> SNAMSARKLFYLGPQGTFTHQAAVNAAQELARFEPQGFDLMPMDDVPQILDAAQHGDGWGIVAWENNVEGYVVPNLDALIDAKDLVGFARVGVNVEFDAYVAQGADPAEARIATAHPHGLAQCKRFIAEHRLSTQPATSNAAACRDLIPGEIAFGPAICGELYDITRIGTAIQDYQGAATDFLVLSPRAEVARLLAKPRAEANVEYESVLTLIPLVTGPGVLANLLDVFRDAGLNMTSFISRPIKGRTGTYSFIVTLDAAPWEERFRDALVEIAEHGDWAKTLAVYPRREHP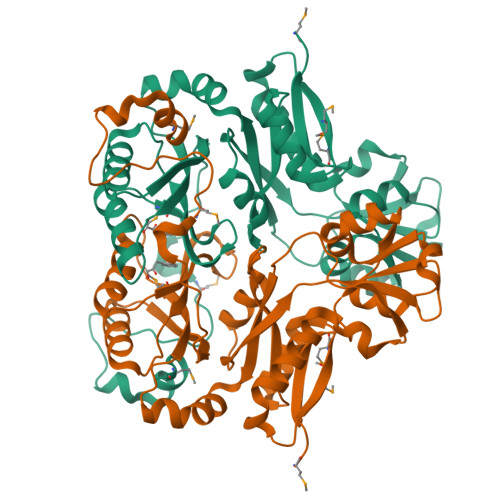NPPVTSWMLPQGGVRLDDSHLPDDWQNDETVRRELMW>MTTIRGDDLSNQITQISGSSSKKEEEKKKQQMLTGVLGLQPTMANHPVLGVFLPKYAKQNGGNVDKTAFRLDLIRMLALHRLNTKTGSD[16x];>MNSKSSARAAIVDTVEAVKKRKYISIEAGTLNNVVEKERKFLKQFLSGRENLRIAARVFTPCELLAPELENLGMLMYRFETDVDNPKILFVGLFFLCSNAFNVSACVRTALTTMYTNSMVDNVLSMINTCKYLEDKVSLFGVTSLVSCGSSCLLSCVMQGNVYDANKENIHGLTVLKEIFLEPDWEPRQHSTQYVYVVHVYKEVLSKLQYGIYVVLTSFQNEDLVVDILRQYFEKERFLFLNYLINSNTTLSYFGSVQRIGRCATEDIKSGFLQYRGITLPVIKLENIFVDLSEKKVFV[5x];>METVYCTFDHKLSLSDISTLCKLMNIVIPIPAHHHLIGSGNLGLYPIVSSNKDYVHIRNVLRTMVVTILQKVEGNQLVLRKPMTGQQYAIKNTGPFPWEKGDTLTLIPPLSTHSEEKLLKLGDWELTVPLVVPTAIAAEINIRLLCIGLIAVHREYNEMQTIIDELCSIQYRDVLIKLPDIVNDKQSMYSMKTACISLSMITAMAPDIVRTYIDRLTLEDHSMLLIKCQELLSKRTTLSTQRCGQLHATDIKDELKKIKSVLTMIDQINSLTNEKTYFVVCDVSADNRMATCIYKN[10x];>[16x]MENWQATEILPKIEAPLNIFNDIKTYTAEQLFDNLRIYFGDDPSRYNISFEALLGIYCNKIEWINFFTTPIAVAANVIRFNDVSRMTLGKVLFFIQLPRVATGNDVTAPKETTIMVAKHSEKHPINISFDLSAACLEHLENTFKNTVIDQILNINALHTVLRSLKNSADSLERGLIHAFMQTLLRKSPPQFIVLTMNENKVHNKQALSRVQRSNMFQSLKNRLLTSLFFLNRNNNSSYIYRILNDMMESVTESILNDTNNYTSKENIPLDGVLLGPIGSIQKLTNILSQYISTQVVSAPISYGHFIMGKENAVTAIAYRAIMADFTQFTVNAGTEQQDTNNKSEIFDKSRAYADLKLNTLKLGDKLVAFDHLHKVYKNTDVNDPLEQSLQLTFFFPLGIYIPTETGFSTMETRVKLNDTMENNLPTSVFFHNKDQVVQRIDFADILPSVCHPIVHDSTIVERLMKNEPLPTGHRFSQLCQLKITRENPTRILQTLYNLYESRQEVPKNTNVLKNELNVEDFYKPDNPTLPTERHPFFDLTYIQKNRATEVLCTPRIMIGNMPLPLAPISFHEARTNQMLEHAKTNSHNYDFTLKIVTESLTSGSYPELAYVIEILVHGNKHAFMILKQVISQCISYWFNMKHILLFCNSFEMIMLISNHMGDELIPGAAFAHYRNLVSLIRLVKRTISISNINEQLCGEPLVNFANALFDGRLFCPFVHTMPRNDTNAKITADDTPLTQNTVRVRNYEISDVQRMNLIDSSVVFTDNDRPSNENTILSKIFYFCVLPALSNNKACGAGVNVKELVLDLFYTEPFICPDDCFQENPISSDVLMSLIREAMGPGYTVANTSSIAKQLFKSLIYINENTKILEVEVSLDPAQRHGNSVHFQSLQHILYNGLCLISPITTLRRYYQPIPFHRFFSDPGICGTMNADIQVFLNTFPHYQRNDGGFPLPPPLALEFYNWQRTPFSVYSAFCPNSLLSIMTLAAMHSKLSPVAIAIQSKSKIHPGFAATLVRTDNFDVECLLYSSRAATSIILDDPTVTAEAKDIVTTYNFTQHLSFVDMGLGFSSTTATANLKRIKSDMGSKIQNLFSAFPIHAFTNTDINTWIRHHVGIEKPNPSEGEALNIITFGGINKNPPSILLHGQQAICEVILTPVTTNINFFKLPHNPRGRESCMMGTDPHNEEAARKALYDHTQTDSDTFAATTNPWASLPGSLGDILYNTAHREQLCYNPKTYSPNAQFFTESDILKTNKMMYKVINEYCMKSNSCLNSDSEIQYSCSEGTDSFVSRPCQFLQNALPLHCSSNQALLESRSKTGNTQISETHYCNYAIGETIPLQLIIESSI;>[12x]MDLKAQSIPFAWLDRDKVQRLTNFLSNLENLENVDLREHPYVTNSCVVREGEDVDELKTLYNTFILWLMYHYVLSKRKPDYNAIWQDITKLQNVVNEYLKSKGLNKGNFENMFTNKEKFESQFSDIHRALLRLGNSIRWGSNVPIDTPYVNLTAEDSSEIENNLQDAEKNMLWYTVYNINDPWDENGYLVTSINKLVYLGKLFVTLNQSWSKLEKVAMSQIVTTQNHLSGHLRKNENFNAVYSQRVLQTPLTGQRVESFLKIITSDYEIIKSSLESYSASKAFSVPENGPHSLMDFASLDGRMPSDLSLPSISIDTKRPSADLARLKISQPKSLDAPLKTQRRHKFPESDSVDNAGGKILIKKETLGGRDVRATTPVSSVSLMSGVEPLSSLTSTNLDLRDKSHGNYRIGPSGILDFGVKLPAEAQSNTGDVDLLQDKTSIRSPSSGITDVVNGLANLNLRQNKSDVSRPWSKNTAANADVFDPVHRLVSEQTGTPFVLNNSDVAGSEAKLTTHSTETGVSPHNVSLIKDLRDKDGFRKQKKLDLLGSWTKEKNDKAIVHSREVTGDSGDATETVTARDSPVLRKTKHANDIFAGLNKKYARDVSRGGKGNSRDLYSGGNAEKKETSGKFNVDKEMTQNEQEPLPNLMEAARNAGEEQYVQAGLGQRVNKILAEFTNLISLGEKGIQDILHNQSGTELKLPTENKLGRESEEANVERILEVSDPQNLFKNFKLQNDLDSVQSPFRLPNADLSRDLDSVSFKDALDVKLPGNGEREIDLALQKVKAGERETSDFKVGQDETLIPTQLMKVETPEEKDDVIEKMVLRIRQDGETDEETVPGPGVAESLGIAAKDKSVIAS

The T = 16 icosahedral HHV-6B capsid structure contains 12 pentons, 150 hexons, and 320 triangular triplexes. Each of the 60 asymmetric units of the HHV-6B capsid contains 16 copies of the major capsid protein (MCP); 16 copies of the smallest capsid protein (SCP), each atop an MCP; five and one-third triplexes (Ta, Tb, Tc, Td, Te, and one-third of Tf); and 12 copies of pU11. As a result, we derived the atomic model of both the HHV-6B capsid and its capsid-associated tegument complex of pU11 tetramer. Beyond the capsid, the helix-rich tegument protein pU11 forms tetramers, bridging the space between the upper domain of the hexon MCP and the triplexes Tb, Td, and Te.

Only the N-terminal one-third of pU11, referred to as pU11nt below, is resolved in the cryoEM density map, indicating the rest of the protein is flexible. A pU11nt tetramer binds atop triplex Tb, Td, or Te, but not Ta, Tc, and Tf. Atop the triplex, four pU11nt subunits cluster into a tetramer in a “VΛ”-shaped, dimer-of-dimers configuration and their subunits can be classified into four types based on their relative locations in the dimer-of-dimers: pU11nt-a-1, pU11nt-a-2, pU11nt-b-1, and pU11nt-b-2. Through this structure, the N-anchor anchors Tri1 and the entire triplex from inside the capsid and beneath the MCP floor region, simultaneously sealing the hole at the local threefold axis where three neighboring MCP P-subdomains encounter one another. Our SCP model encompasses residues 23–83 of the 89 residue-long SCP and consists of three α-helices and two connecting loops, folded into a triangular spiral with the N-terminal helix (H1) pointing outwards. Our model shows that SCP’s helix H3 contributes the largest number of interacting residues between SCP and MCP, inserting itself into a groove in the upper domain of MCP. CATC exists as a group-of-four subunits in HHV-6B, but as a group-of-two subunits in MCMV and a group-of-three subunits in HCMV; it is arranged in a “VΛ” formation in HHV-6B, “Λ” in MCMV, and “Δ” in HCMV. Conceivably, the rigidity of the helix-rich pU11nt tetramer may have made it impossible to extend in order to span a longer distance, or to shrink in order to prevent clashes, thus explaining the absence of pU11 above triplex Ta in HHV-6B.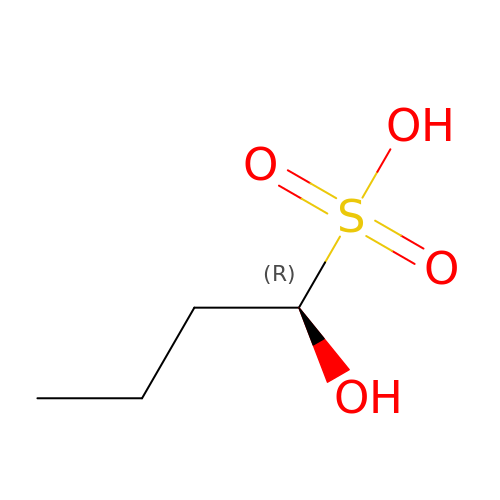(1R)-1-hydroxybutane-1-sulfonic acid | C4 H10 O4 S | KMBRJVMBQNMRDM-SCSAIBSYSA-N> YRL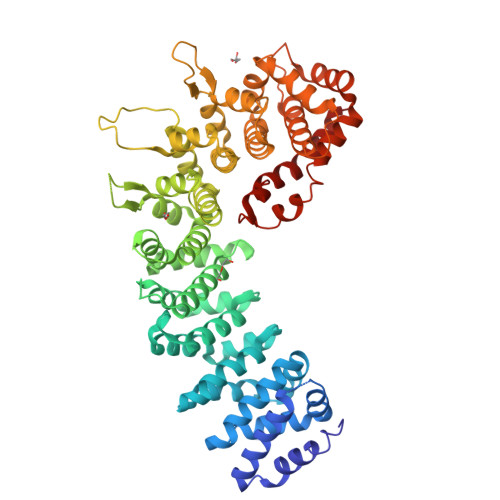EVGIQAMEHLIHVLQTDRSDSEIIGYALDTLYNIISNEEEEEVEENSTRQSEDLGSQFTEIFIKQQENVTLLLSLLEEFDFHVRWPGVKLLTSLLKQLGPQVQQIILVSPMGVSRLMDLLADSREVIRNDGVLLLQALTRSNGAIQKIVAFENAFERLLDIISEEGNSDGGIVVEDCLILLQNLLKNNNSNQNFFKEGSYIQRMKPWFEVGDENSGWSAQKVTNLHLMLQLVRVLVSPTNPPGATSSCQKAMFQCGLLQQLCTILMATGVPADILTETINTVSEVIRGCQVNQDYFASVNAPSNPPRPAIVVLLMSMVNERQPFVLRCAVLYCFQCFLYKNQKGQGEIVSTLLPSTIDATGNSVSAGQLLCGGLFSTDSLSNWCAAVALAHALQENATQKEQLLRVQLATSIGNPPVSLLQQCTNILSQGSKIQTRVGLLMLLCTWLSNCPIAVTHFLHNSANVPFLTGQIAENLGEEEQLVQGLCALLLGISIYFNDNSLESYMKEKLKQLIEKRIGKENFIEKLGFISKHELYSRASQKPQPNFPSPEYMIFDHEFTKLVKELEGVITKAIY>GSALQDRPIKNTICLFDVDETLTPARRAVTPEMLMLLSQLRHKCAIGYVGGSNLAKQQEQLGTGATDVTSLFDFCFPENGLMAFRLGKPLASTSFIEWIGEEKYQKLVNFILRYFADLQLPKKRGTFIEFRNGMINVSPIGRNASVEERNEFEAYDKEHHIRTDMVNALKKEFPDYGLTYSIGGQISFDVFPTGWDKTYCLRHVEAEKEI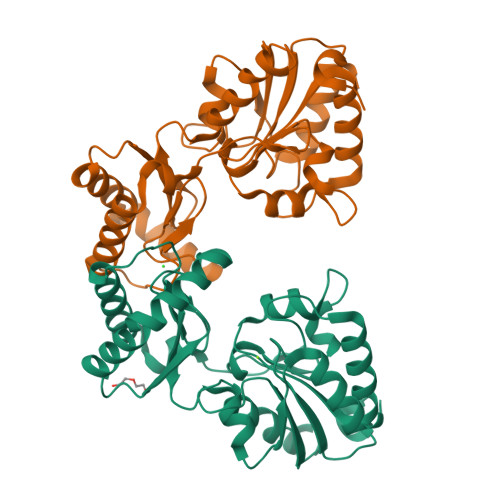SGVEYTTIHFFGDKCFPGGNDYEIYSDPRTIGHSVHGPEDTMKQLKELFQL[4x]> SPILGYWKIKGLVQPTRLLLEYLEEKYEEHLYERDEGDKWRNKKFELGLEFPNLPYYIDGDVKLTQSMAIIRYIADKHNMLGGCPKERAEISMLEGAVLDIRYGVSRIAYSKDFETLKVD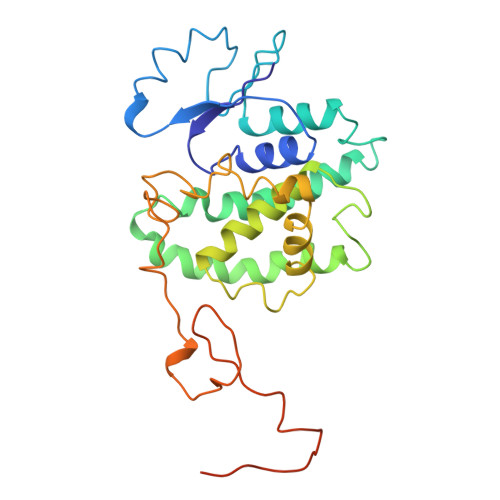FLSKLPEMLKMFEDRLCHKTYLNGDHVTHPDFMLYDALDVVLYMDPMCLDAFPKLVCFKKRIEAIPQIDKYLKSSKYIAWPLQGWQATFGGGDHPPKSDLVPRGSRRASVGSRMHYPGAFTYSPTPVTSGIGIGMSAMGSATRYHTYLPPPYPGEFIVID(1R,2R)-2-fluorocyclopentyl {(2R,4S,6S,12Z,13aS,14aR,16aS)-2-[(7-methoxy-3-methylquinoxalin-2-yl)oxy]-14a-[(1-methylcyclopropane-1-sulfonyl)carbamoyl]-5,16-dioxo-1,2,3,5,6,7,8,9,10,11,13a,14,14a,15,16,16a-hexadecahydrocyclopropa[e]pyrrolo[1,2-a][1,4]diazacyclopentadecin-6-yl}carbamate 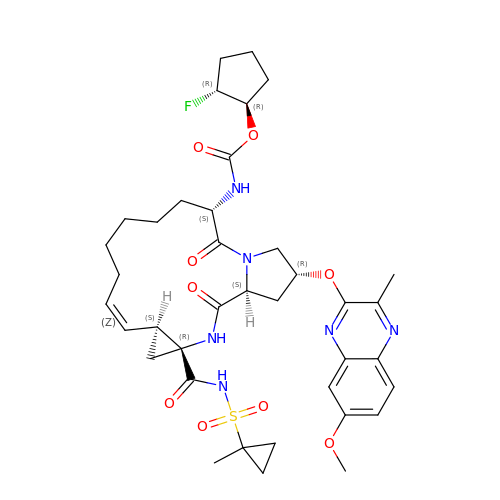| C38 H49 F N6 O9 S | TURVLKLYHQZYDB-LRIBJDGDSA-N> MAVPGYYELYRRSTIGNSLVDALDTLISDGRIEASLAMRVLETFDKVVAETLKDNTQSKLTVKGNLDTYGFCDDVWTFIVKNC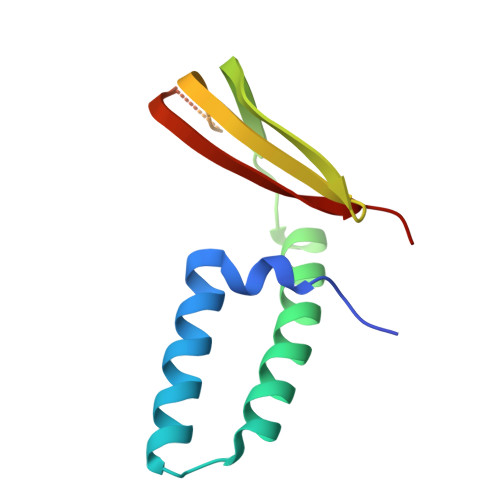QVTVEDSHRDASQNGSGDSQSVISVDKLRIVACNSKKSE> EETVTCLQMTVYHPGQLQCGIFQSISFNREKLPSSEVVKFGRNSNICHYTFQDKQ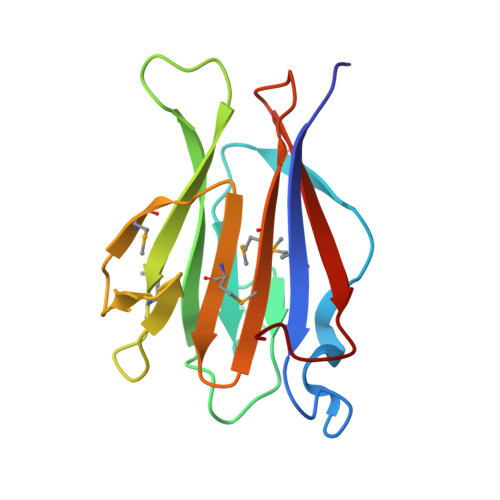VSRVQFSLQLFKKFNSSVLSFEIKNMSKKTNLIVDSRELGYLNKMDLPYRCMVRFGEYQFLMEKEDGESLEFFETQFILSPRSLLQ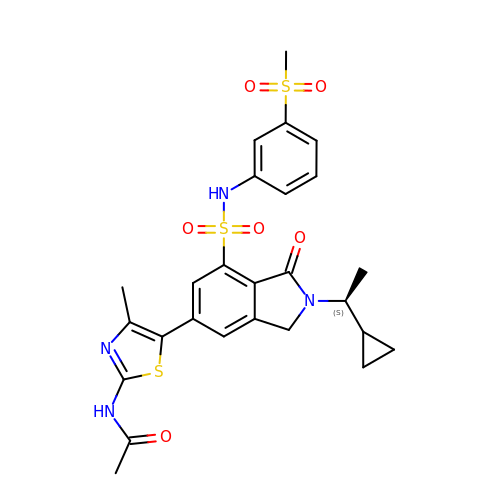N-[5-[2-[(1S)-1-cyclopropylethyl]-7-[(3-methylsulfonylphenyl)sulfamoyl]-1-oxidanylidene-3H-isoindol-5-yl]-4-methyl-1,3-thiazol-2-yl]ethanamide | C26 H28 N4 O6 S3 | CZHFAPKIYABWLB-HNNXBMFYSA-N Lsr2 from M. tuberculosis is a small, basic protein (Mr = 12.1 kDa, pI = 10) that is highly conserved in mycobacteria and related actinobacteria. Lsr2 is a DNA-binding protein that likely influences the organization of bacterial chromatin and gene regulation by binding to AT-rich segments of DNA. The Lsr2 dimerization domain forms a compact homodimeric α/β structure. The dimer forms a 4-stranded anti-parallel β-sheet such that the helices are arranged in an antiparallel fashion and are on the same side of the β-sheet.

Here, we report the structure of the N-terminal dimerization domain of Lsr2 solved by X-ray crystallography at 1.73 Å resolution using ab initio methods. Crystals grew from one of these constructs (Nterm2) after a few days but this was dependent on “maturation” of the protein sample (by some unknown process) over a long period of time. In retrospect, this “maturation” process amounted to degradation of Lsr2 at Lys-4 to generate a truncation product with Lys-4 as the new N-terminal residue. The structure in the monoclinic space group P21 was solved at 1.8 Å using the latest version of the ARCIMBOLDO program. A 14-residue long model polyalanine alpha-helix was used as the search fragment to arrive at the ab initio solution. We subsequently learned that these absent residues at the N-terminus had been cleaved by contaminating proteases in the case of the P21 crystals. The monoclinic crystal structure reveals a linear chain of dimers formed by crystallographic symmetry. The N-terminal end of each dimer forms a single ß-strand (ß0) that is then paired with the N-terminal strand of a neighboring dimer to form the linear oligomer chain. The oligomer is not only stabilized by interstrand H-bonds, but also by a network of polar interactions between Lys-4 (the new N-terminus after truncation) and its oligomeric neighbor.

>[2x]MAKKVTVTLVDDFDGSGAADETVEFGLDGVTYEIDLSTKNATKLRGDLKQWVAAGRRVGGR> KNADSYAKKPHISALNAPQLDQRYKNEFTIGAAVEPYQLQNEKDVQMLKRHFNSIVAENVMKPISIQPEEGKFNFEQADRIVKFAKANGMDIRFHTLVWHSQVPQWFFL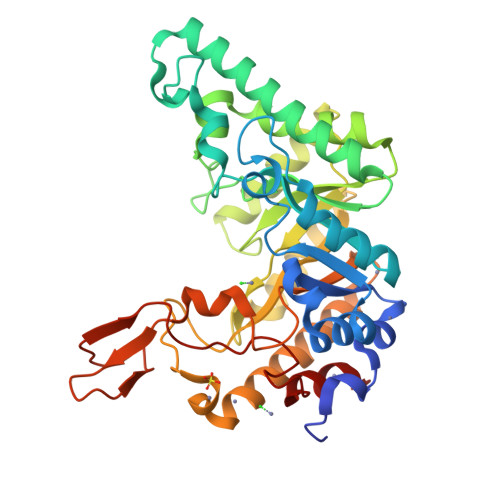DKEGKPMVNETDPVKREQNKQLLLKRLETHIKTIVERYKDDIKYWDVVNAVVGDDGKLRNSPWYQIAGIDYIKVAFQAARKYGGDNIKLYMNDYNTEVEPKRTALYNLVKQLKEEGVPIDGIGHQSHIQIGWPSEAEIEKTINMFAALGLDNQITALDVSMYGWPPRAYPTYDAIPKQKFLDQAARYDRLFKLYEKLSDKISNVTFWGIADNHTWLDSRADVYYDANGNVVVDPNAPYAKVEKGKGKDAPFVFGPDYKVKPAYWAIIDHK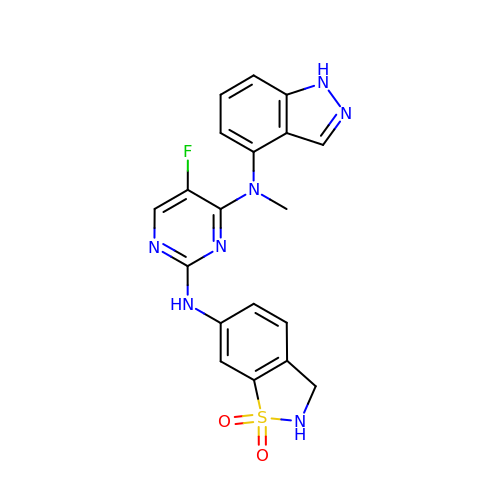N~2~-(1,1-dioxido-2,3-dihydro-1,2-benzothiazol-6-yl)-5-fluoro-N~4~-(1H-indazol-4-yl)-N~4~-methylpyrimidine-2,4-diamine | C19 H16 F N7 O2 S | AKKNJEBKJABIRC-UHFFFAOYSA-N> MTGGMKPPARKPRILNSDGSSNITRLGLEKRGWLDDHYHDLLTVSWPVFITLITGLYLVTNALFALAYLACGDVIENARPGSFTDAFFFSVQTMATIGYGKLIPIGPLANTLVTLEALCGMLGLAVAARLIYARFTRPT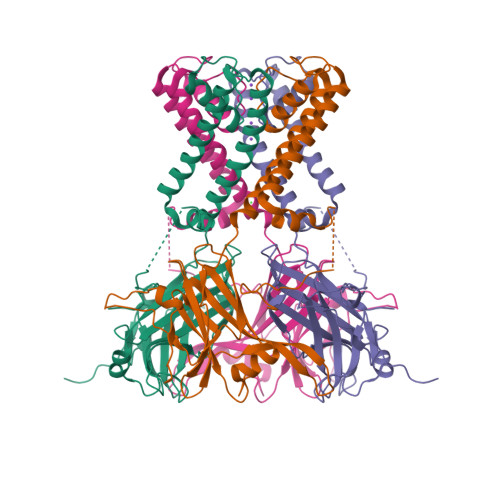AGVLFSSRMVISDFEGKPTLMMRLANLRIEQIIEADVHLVLVRSEISQEGMVFRRFHDLTLTRSRSPIFSLSWTVMHPIDHHSPIYGETDETLRNSHSEFLVLFTGHHEAFAQNVHARHAYSCDEIIWGGHFVDVFTTLPDGRRALDLGKFHEIAQHHHHHH>[2x]MANLLKTVVTGCSCPFLSNLGSCKVLPGKKNFLRAFHTHRILWCKAPVKPGIPYKQLTVGVPKEIFQNEKRVALSPAGVQALVKQGFNVVVESGAGEASKFSDDHYRAAGAQIQGAKEVLASDLVVKVRAPMLNPTLGIHEADLLKTSGTLISFIYPAQNPDLLNKLSKRNTTVLAMDQVPRVTIAQGYDALSSMANIAGYKAVVLAANHFGRFFTGQITAAGKVPPAKILIVGGGVAGLASAGAAKSMGAIVRGFDTRAAALEQFKSLGAEPLEVDLKESGEGQGGYAKEMSKEFIEAEMKLFAQQCKEVDILISTALIPGKKAPILFNKEMIESMKEGSVVVDLAAEAGGNFETTKPGELYVHKGITHIGYTDLPSRMATQASTLYSNNITKLLKAISPDKDNFYFEVKDDFDFGTMGHVIRGTVVMKDGQVIFPAPTPKNIPQGAPVKQKTVAELEAEKAATITPFRKTMTSASVYTAGLTGILGLGIAAPNLAFSQMVTTFGLAGIVGYHTVWGVTPALHSPLMSVTNAISGLTAVGGLVLMGGHLYPSTTSQGLAALATFISSVNIAGGFLVTQRMLDMFKRPTDPPEYNYLYLLPAGTFVGGYLASLYSGYNIEQIMYLGSGLCCVGALAGLSTQGTARLGNALGMIGVAGGLAATLGGLKPCPELLAQMSGAMALGGTIGLTIAKRIQISDLPQLVAAFHSLV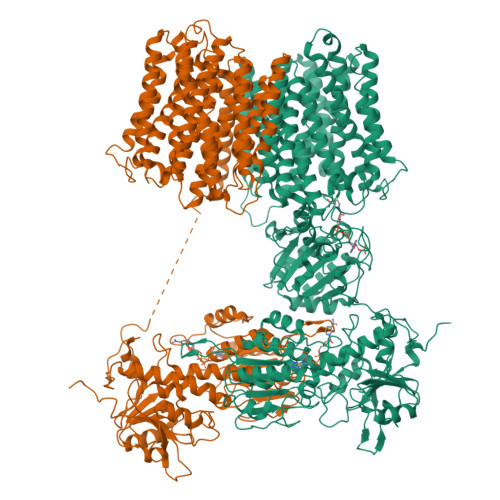GLAAVLTCIAEYIIEYPHFATDAAANLTKIVAYLGTYIGGVTFSGSLVAYGKLQGILKSAPLLLPGRHLLNAGLLAASVGGIIPFMMDPSFTTGITCLGSVSALSAVMGVTLTAAIGGADMPVVITVLNSYSGWALCAEGFLLNNNLLTIVGALIGSSGAILSYIMCVAMNRSLANVILGGYGTTSTAGGKPMEISGTHTEINLDNAIDMIREANSIIITPGYGLCAAKAQYPIADLVKMLSEQGKKVRFGIHPVAGRMPGQLNVLLAEAGVPYDIVLEMDEINHDFPDTDLVLVIGANDTVNSAAQEDPNSIIAGMPVLEVWKSKQVIVMKRSLGVGYAAVDNPIFYKPNTAMLLGDAKKTCDALQAKVRESYQK>TEATRKHVQQLMKVFRAIDFDFTKKAFYLHRAKYGVQNQLRNPLYLKAMSLPRSAKLSQPCLNKMIDEVNDLESTFYAGF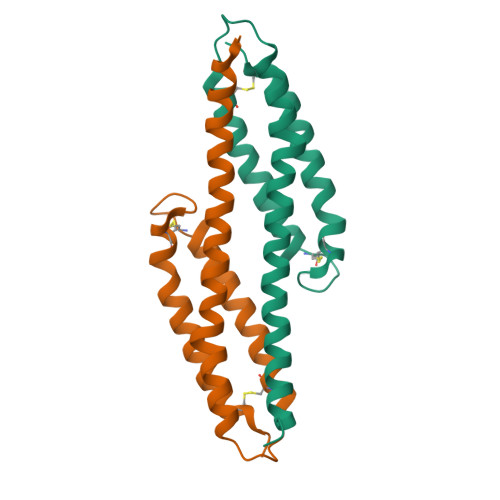SFNCHDHDQYSMDCLEAAEPTYLDGLKKLAASTEQCLVQK[3x]> GSNPAEELAAAAQRGDVIAILQQALETNSFRLLFQPVISLRGDSHENYEVLLRLLNPQGQEVPPAEFLHAAKEAGLAEKIDRWVILNSIKLLAEHRAKGHQTKLFVHLSSASLQDPGLLPW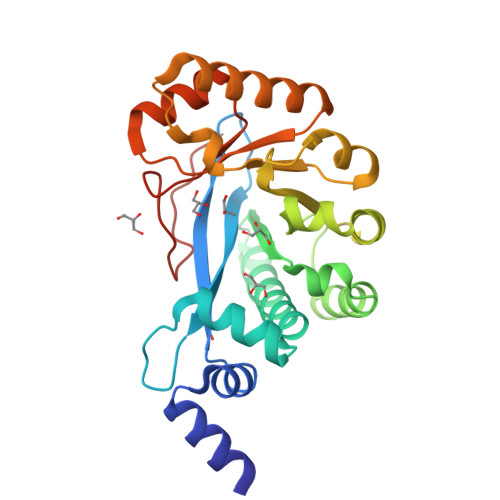LGVALKAARLPPESLVFQISEADATSYLKQAKQLTQGLATLHCQAAISQFGCSLNPFNALKHLTVQFIKIDGSFVQDLNQVENQEILKGLIAELHEQQKLSIVPFVESASVLATLWQAGATYIQGYYLQGPSQAMDYDFSSGDE>MALPSVTALEIENYAFPPTVKPPGSTNNFFLGGAGERGIQIQDKFVKFTAIGVYLQDIAVPYLAEKWKARSAHELTDTVPFFRDIVTGPFEKFMRVTMILPLTGHQYSEKVSENCVAIWKSLGIYTDEEAKAIDKFVSVFKDETFPPGSSILFTVSPKGLGSLTISFSKDGSIPEVETAVIENKLLSQAVL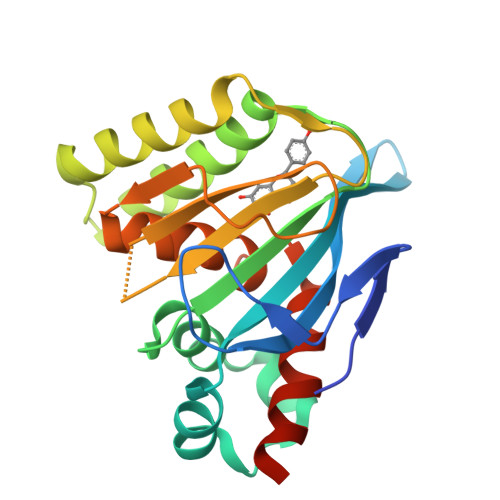ESMIGAHGVSPAAKQSLASRLSKLFKEGGNANN[8x]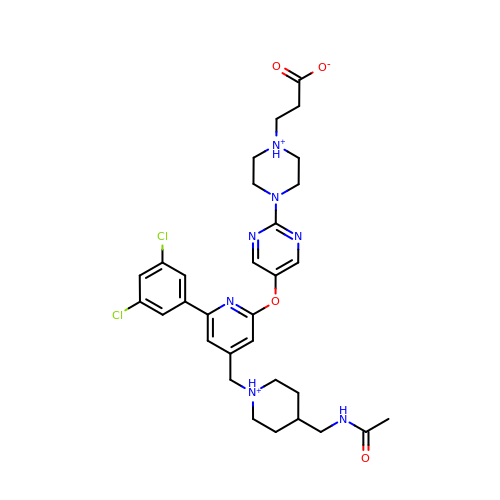3-[4-[5-[4-[[4-(acetamidomethyl)piperidin-1-ium-1-yl]methyl]-6-[3,5-bis(chloranyl)phenyl]pyridin-2-yl]oxypyrimidin-2-yl]piperazin-1-ium-1-yl]propanoate | C31 H38 Cl2 N7 O4 | DIZGFRSKRZZKAK-UHFFFAOYSA-O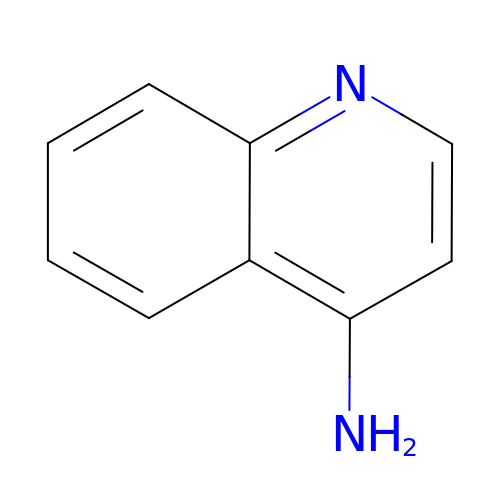quinolin-4-amine | C9 H8 N2 | FQYRLEXKXQRZDH-UHFFFAOYSA-N3-[3,5-bis(fluoranyl)-4-[3-(hydroxymethyl)phenyl]phenyl]benzo[f]benzotriazole-4,9-dione | C23 H13 F2 N3 O3 | 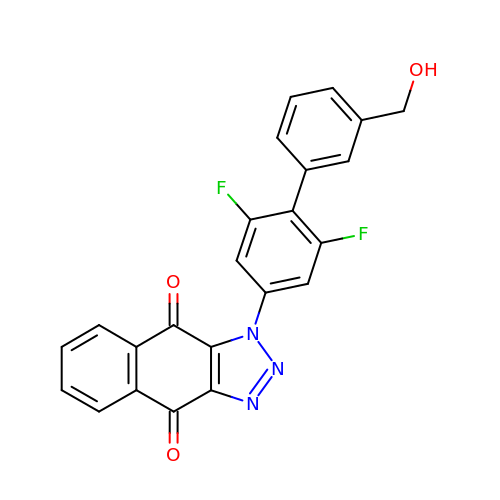INHJBTZMBKOVDA-UHFFFAOYSA-N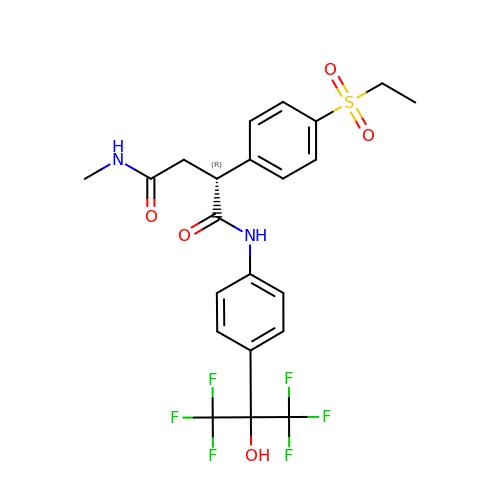(2~{R})-2-(4-ethylsulfonylphenyl)-~{N}-[4-[1,1,1,3,3,3-hexakis(fluoranyl)-2-oxidanyl-propan-2-yl]phenyl]-~{N}'-methyl-butanediamide | C22 H22 F6 N2 O5 S | FQOWZQYVIFDJJK-QGZVFWFLSA-N>[2x]MNNPADAGINLNYLANVRPSSRQLAWQRMEMYAFLHFGMNTMTDREWGLGHEDPALFNPRNVDVDQWMDALVAGGMAGVILTCKHHDGFCLWPSRLTRHTVASSPWREGKGDLVREVSESARRHGLKFGVYLSPWDRTEESYGKGKAYDDFYVGQLTELLTQYGPIFSVWLAGANGEGKNGKTQYYDWDRYYNVIRSLQPDAVISV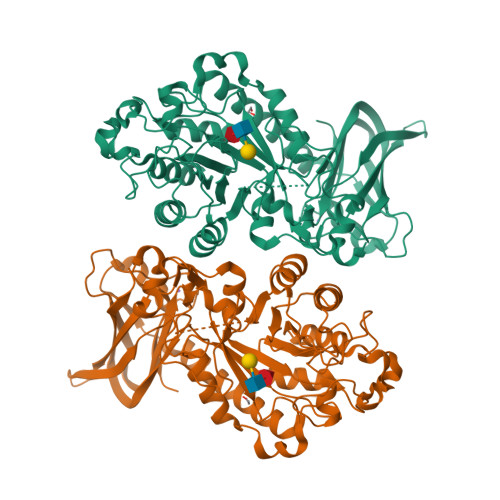CGPDVRWAGNAAGHVRDNEWSVVPRRLRSAELTMEKSQQEDDASFATTVSSQDDDLGSREAVAGYGDNVCWYPAEVDTSIRPGWFYHQSEDDKVMSADQLFDLWLSAVGGNSSLLLNIPPSPEGLLAEPDVQSLKGLGRRVSEFREALASVRCEARTSSASAAAAHLVDGNRDTFWRPDADDAAPAITLTLPQPTTINAIVIEEAIEHGQRIEHLRVTGALPDGTERVLGQAGTVGYRRILRFDDVEVSSVTLHVDGSRLAPMISRAAAVRI>[2x]SQLVECVPNFSEG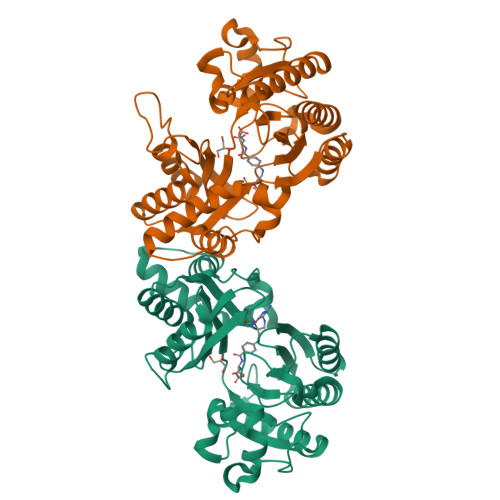KNQEVIDAISRAVAQTPGCVLLDVDSGPSTNRTVYTFVGRPEDVVEGALNAARAAYQLIDMSRHHGEHPRMGALDVCPFIPVRGVTMDECVRCAQAFGQRLAEELGVPVYLYGEAARTAGRQSLPALRAGEYEALPEKLKQAEWAPDFGPSAFVPSWGATVAGARKFLLAFNINLLSTREQAHRIALDLREQGRGKDQPGRLKKVQAIGWYLDEKNLAQVSTNLLDFEVTGLHTVFEETCREAQELSLPVVGSQLVGLVPLKALLDAAAFYCEKENLFLLQDEHRIRLVVNRLGLDSLAPFKPKERIIEYLV> GSHMSKSLKKLVEESREKNQPEVDMSDR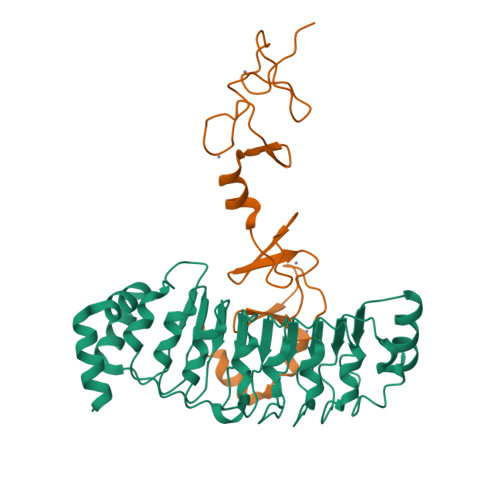GISNMLDVNGLFTLSHITQLVLSHNKLTMVPPNIAELKNLEVLNFFNNQIEELPTQISSLQKLKHLNLGMNRLNTLPRGFGSLPALEVLDLTYNNLSENSLPGNFFYLTTLRALYLSDNDFEILPPDIGKLTKLQILSLRDNDLISLPKEIGELTQLKELHIQGNRLTVLPPELGNLDLTGQKQVFKAENNPWVTPIADQFQLGVSHVFEYIRSETYKYLYGRHMQANPEPPKKNNDKSKKISRKPLAAKNR;> GSPEGVPICGACRRPIEGRVVNAMGKQWHVEHFVCAKCEKPFLGHRHYERKGLAYCETHYNQLFGDVCFHCNRVIEGDVVSALNKAWCVNCFACSTCNTKLTLKNKFVEFDMKPVCKKCYEKFPLELKKRLKKLAETLGRK>[2x]GSMVTVEEVRKAQRAEGPATVLAIGTATPSNCVDQATYPDYYFRITNSEHKTELKEKFQRMCDKSMIKKRYMYLTEEILKENPTVCEYMAPSLDARQDMVVVEVPRLGKEAATKAIKEWGQPKSKITHLVFCTTSGVDMPGADYQLTKLLGLRPYVKRLMMYQQGCFAGGTVLRLAKDLAENNKGARVLVVCSEITAVTFRGPSDTHLDSLVGQALFGDGAAAVIIGADPLPEVEKPLFELVSAAQTILPDSDGAIDGHLREVGLTFHLLKDVPGLISKNIEKSLNEAFKPIGISDWNSLFWIAHPGGPAILDQVESKLALKPEKLEATRQVLSNYGNMSSACVLFILDEVRRKSTEKGLRTTGEGLEWGVLFGFGPGLTVETVVLHSVA

Type III PKS catalysis involves the loading of a CoA-tethered substrate onto an active-site cysteine followed by chain elongation via iterative decarboxylative Claisen condensations of malonyl-CoA. Linear poly­ketide intermediates undergo a terminal intramolecular cyclization reaction to produce the final cyclic polyketide product. The five-layered αβαβα topology of secondary-structural elements of each monomer is consistent with the ‘thiolase fold’ originally observed in thiolase and present in all known structures of type III PKSs.

BLAST searches and analysis of the apple genome showed that one of the cDNAs was >96% identical in amino-acid sequence to chalcone synthases from Malus. The crystallographic model of MdCHS2 contained 774 out of 778 residues. The active-site cavity of MdCHS2 is conserved and isomorphous with the previously characterized cavity of M. sativa CHS. The gatekeeper residues, Phe215 and Phe265 in MdCHS2, separate the CoA tunnel from the internal active-site cavity and affect substrate selectivity by acting as a steric gate during substrate binding. Residues of the MdCHS2 pocket include Ser133, Glu192, Thr194, Thr197, Gly216 and Ser338. Ser338 of MdCHS2 resides at the intersection of the coumaroyl-binding pocket and elongation/cyclization cavity and stabilizes the conformation of elongated polyketide intermediates. Nonetheless, displacement of the region B loop is not observed in any available CHS structures.5-acetamido-2,6-anhydro-3,4,5-trideoxy-3-fluoro-D-erythro-L-gluco-nononic 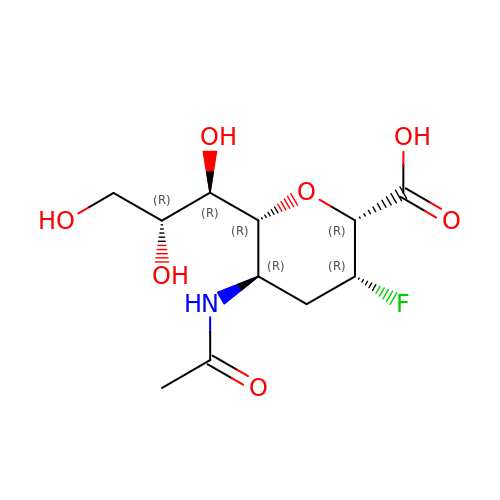acid | C11 H18 F N O7 | AUOXJUOLLXNWIV-MMDZMLKVSA-N ACARBOSE DERIVED 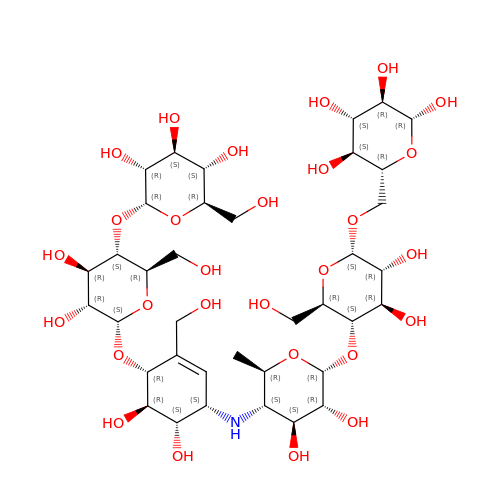HEXASACCHARIDE | C37 H63 N O28 | MBNITLCAVXHYER-DHAMQIFDSA-N>MTKYALVGDVGGTNARLALCDIASGEISQAKTYSGLDYPSLEAVIRVYLEEHKVEVKDGCIAIACPITGDWVAMTNHTWAFSIAEMKKNLGFSHLEIINDFTAVSMAIPMLKKEHLIQFGGAEPVEGKPIAVYGAGTGLGVAHLVHVDKRWVSLPGEGGHVDFAPNSEEEAIILEILRAEIGHVSAERVLSGPGLVNLYRAIVKADNRLPENLKPKDITERALADSCTDCRRALSLFCVIMGRFGGNLALNLGTFGGVFIAGGIVPRFLEFFKASGFRAAFEDKGRFKEYVHDIPVYLIVHDNPGLLGSGAHLRQTLGHILHHHHHH[2x]

Glucokinase (GLK) catalyzes the first reaction in the glycolytic pathway and is a target for regulation in a wide range of organisms. Group II GLKs are ATP-dependent enzymes that lack the classical repressor open reading frame kinase (ROK) sequence motif and contain more than 50 partial and complete protein sequences, including Escherichia coli GLK (ecGLK; Titgemeyer et al., 1994; Meyer et al., 1997). To date, there are no ecGLK structures reported together with the other substrate ATP or the product ADP. This work presents the structure of apo ecGLK bound with phosphate and the structure of ecGLK in complex with both glucose and phosphate, implying a role for phosphate in regulation of the GLK activity. In the ternary complex, phosphate is bound adjacent to glucose, and the B factors for the α4, α5 and α9 helices were further reduced, while r.m.s.d. spikes were observed at the end of the β10 sheet and within the α6 helix of the β-domain. This structural characterization suggests that phosphate could influence the activity of GLK by altering glucose binding and modulating interactions with a loop-interacting regulatory protein.

A ternary complex consisting of GLK, glucose and phosphate is also reported in this work. The crystals of the phosphate-bound glucose–ecGLK complex were obtained by soaking ecGLK with 5 mM glucose and were grown in 100 mM bis-Tris pH 6.5, 200 mM magnesium chloride, 25%(w/v) PEG 3350. The crystal structure was determined by molecular replacement and refined to an R factor of 0.2034 (Rfree = 0.2580) at a resolution of 2.54 Å. The small and large domains retain the α-helices and β-sheets found in phosphate-bound ecGLK while there are domain shifts to account for the glucose binding. The small domain shifts down, closing the binding cleft, and the large domain maintains its relative position with slight shifts into the center of ecGLK. The phosphate-bound glucose–ecGLK complex crystallizes in a more highly ordered space group (P212121) compared with the phosphate-free form (P1211), suggesting that phosphate binding stabilizes the conformation of ecGLK. The phosphate binding stabilizes Arg286 and forms hydrogen bonds to the O2 and O4 of phosphate in chain B. This process reinforces the enzyme structure, lowers its flexibility and may improve glucose binding. In the phosphate-free structure, the O atom of Glu187 forms hydrogen bonds to both glucose and water, while in the phosphate-bound complex it forms a new hydrogen bond to Arg286 NH2.> MERNKLARQIIDTCLEMTRLGLNQGTAGQVSVRYQDGMLITPTGIPYEKLTESHIVFIDGNGKHEEGKLPSSEWRFHMAAYQSRPDANAVVH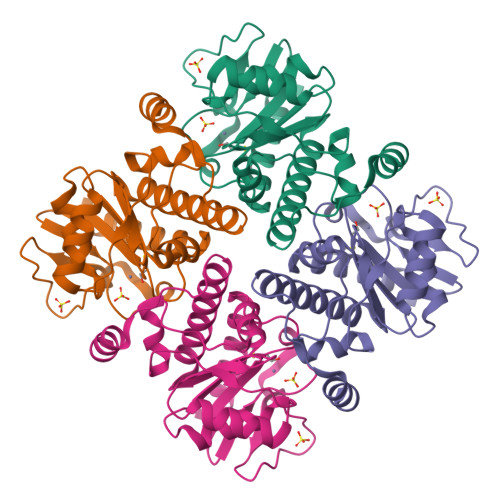NHAVHCTAVSILNRSIPAIHYMIAAAGGNSIPCAPYATFGTRELSEHVALALKNRKATLLQHHGLIACEVNLEKALWLAHEVEVLAQLYLTTLAITDPVPVLSDEEIAVVLEKFKTFGLRIEE>GPLGSSQIPASEQETLVRPKPLLLKLLKSVGAQKDTYTMKEVLFYLGQYIMTKRLYDAAQQHIVYCSNDLLGDLF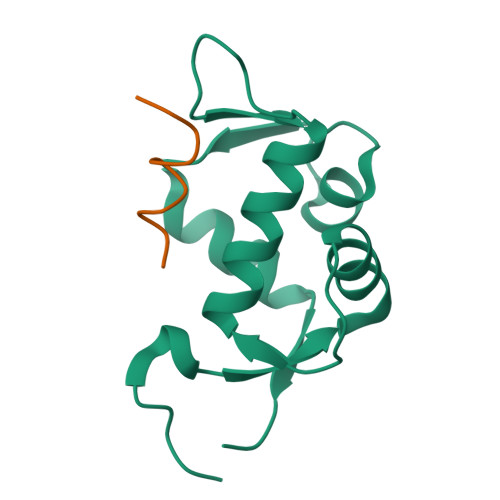GVPSFSVKEHRKIYTMIYRNLVVVNQQESSDSGTSVSEN[4x]>[4x]MFEARLVQGSILKKVLEALKDLINEACWDISSSGVNLQSMDSSHVSLVQLTLRSEGFDTYRCDRNLAMGVNLTSMSKILKCAGNEDIITLRAEDNADTLALVFEAPNQEKVSDYEMKLMDLDVEQLGIPEQEYSCVVKMPSGEFARICRDLSHIGDAVVI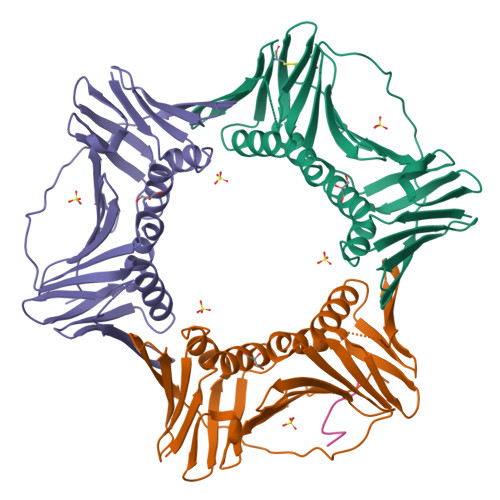SCAKDGVKFSASGELGNGNIKLSQTSNVDKEEEAVTIEMNEPVQLTFALRYLNFFTKATPLSSTVTLSMSADVPLVVEYKIADMGHLKYYLAPKIEDEEGSLEHHHHHH;>[2x]NEILQTLLDLFFPGYSK>ETGDHSRSLKRANLANTSITCNDGSHAGFYLRKHPSSKKWIVLLEGGWHCFDVRSCRSRWMRLRHLMTSSQWPETRDVGGILSPHPEENPYWHNANHVLIPYCSSDSWSGTRTEPDTSDRENSWRFMGALILRQVIAELIPVGLGRVPGGELMLVGSSAGGMGVMLNLDRIRDFLVNEKKLQITVRGVSDSGWFLDREPYTPAAVASNEAVRQGWKLWQGLLPEECTKSYPTEPWRCYYGYRLYPTLKTPLFVFQWLFDEAQMRVDNVGAPVTPQQWNYIHEMGGALRSSLDNVSAVFAPSCIGHGVLFKRDWVN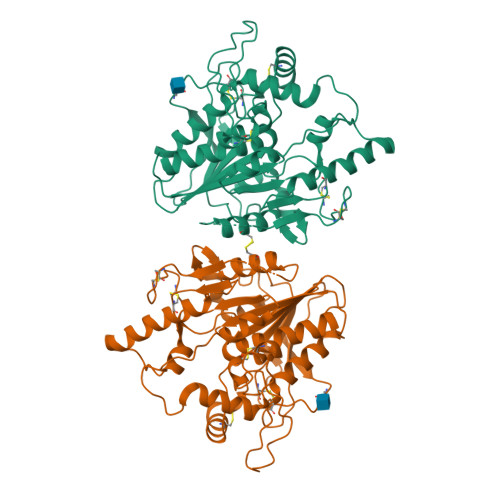IKIDDISLPSALRCWEHSTRSGNNNGCGLRLLERCSWPQCNHSCPTGTHHHHHHHHHH[2x]> GMVLTLSDLEKGYDKNLNQLSLSFLNLRDNDIPLLCEFLQNHPAITSLDLSHNDITANGVKLFVNKTSVSSLNISHNNIGPEGAQWLSEDNHITTLDVSFNEIGDEGVKALAANAKLITLYALYNKITKVGAGYLAQSNLKKIDLCFNSLEDEGVIALASNINIKELIASACDVSDIGAIELAKNNQLTLLILGKNAITDKSTLHFANNTSLSTLHLGSNQITAAGKKILETNTRITDLDLIGNPIEVHETDELNYSKKSPDSHSVFKFLQKFTF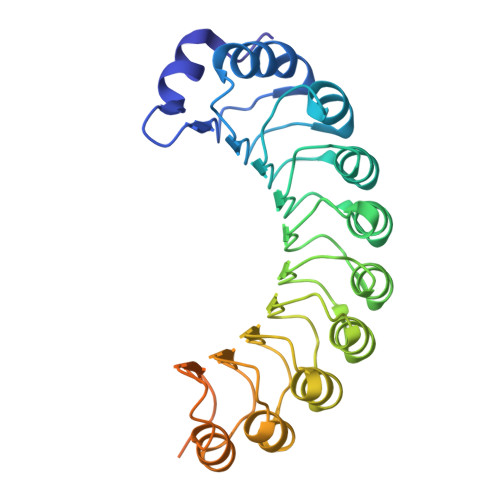LSCMSPCQETAESDKGLNKKPN> SKGLQIRVQGLDEAQEFYELESKADGQLLLSDVFRRINLIESDYFGLEFQNLQMNWVWLDPSKLIVKQVRRPMNTLFRLSVKFFPPDPGQLQEEFTRYLFSLQIKRDLLDGRLSCTENTAALLASHLVQSEIGDYDDLADREFLKMNKLLPCQEHVQEKIMELHRRHTGQTPAESDFQVLEIARKLEMFGVRFHPAADREGTKINLAVAHMGLQVFQGHTKINTFNWSKIRKLSFKRKRFLIKLHPEVHGPHQDTLEFLMGSRDQCKIFWKNCVEHHSFFRLLDQPQPKSKAIFFSRGSSFRYSGRTQKQLVEYVRDSGLRRTPYQRRNSKIR

FARP1 (FERM, RhoGEF and pleckstrin domain-containing protein 1) and its close homolog FARP2 were identified as guanine nucleotide exchange factors (GEFs) for RhoGTPases that play regulatory roles in neuronal development. FARP1 and FARP2 share a conserved domain architecture, containing a N-terminal 4.1, ezrin, radixin and moesin (FERM) domain, which is followed by a long linker (~200 residues) that connects to a Dbl-homology (DH) domain and two pleckstrin homology (PH) domains. We determined crystal structures of the FERM domains of zebrafish FARP1 (zfFARP1), mouse FARP2 (mFARP2) and zebrafish FARP2 (zfFARP2). As expected from their high degree of sequence identity (>60%), the structures of these FERM domains are very similar to one another, with root mean square deviations within 1.0 Å.

The corresponding site in the FERM domains of FARP1 and FARP2 contains a negatively charged residue (Asp97, Glu100 and Asp107 in zfFARP1, mFARP2 and zfFARP2, respectively), suggesting that it cannot serve as a phosphatidylinositol binding site in these FERM domains. In particular, the FERM domains of FARP1 and FARP2 contain a Lys-Arg-Lys-Arg (KRKR) motif in the loop connecting strands β5 to β6 in the F3 subdomain, which is highly conserved in FARP1/2 from different species. Overall, the surface of these FERM domains show highly polarized surface electrostatic potential, with one side positively charged while the opposite side negatively charged. Interestingly, both the FERM domains of mFARP2 and zfFARP2 form similar head-to-tail packing patterns in the crystal lattices, as a result of interactions between the positively charged and the negatively charged faces of the proteins. These packing patterns lead to a linear array of the FERM molecules, which may cause the oligomerization and precipitation of the proteins. The first arginine residue in the KRKR motif (Arg277) in the FERM domain of mFARP2 makes a salt bridge with Asp216 from the neighboring protomer in the linear array. An equivalent salt bridge (Arg284-Asp223) is also present in the structure of the FERM domain of zfFARP2. The linear packing of the FERM domains of mFARP2 and zfFARP2 in our crystal structures suggest a potential mechanism for the oligomerization of these FERM domains. The KRKR motif in the FERM domains responsible for phospholipid binding is buried in the oligomerization interface. We speculate that the oligomerization, if occurs in the cell, could be a mechanism for regulating membrane targeting of FARP1 and FARP2.>MIVKRGDVYFADLSPVVGSEQGGVRPVLVIQNDIGNRFSPTAIVAAITAQIQKAKLPTHVEIDAKRYGFERDSVILLEQIRTIDKQRLTDKITHLDDEMMDKVDEALQISLALIDF[4x];>[2x]SMSESSARTEMKISLPENLVAELDGVAMREKRSRNELISQAVRAYVSERTTRHNRDLMRRGYMEMA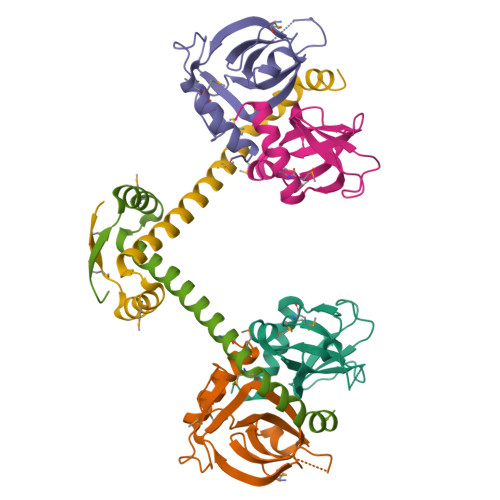KINLNISSEAHFAECEAETTVERLVSGG> GQQVCPNYVMLRSSVTTKVVRNVVEYQIRTGGFFSCLAMLRPLQYAKRERLLGQRNLERISTRDILQTRDLHSLCMPTPDAPMSNHQASTMRELICSYFKVDHADGLKYIPMDERYSPSSLARLFTMGMAGLHITTEPSYKRVPIMHLAADLDCMTLALPYMITLDGDTVVPVAPTLSAEQLLDDGLKGLACMDISYGCEVDANSRPAGDQSMDSSRCINELYCEETAEAICVLKTCLVLNCMQFKLEMDDLAHNAAELDKIQMMIPFSERVFRMASSFATIDAQCFRFCVMMKDKNLKIDMRETTRLWTRSASDDSVATSSLSISLDRGRWVAADASDARLLVFPIRV

The mammalian orthoreovirus (reovirus) σNS protein is required for formation of replication compartments that support viral genome replication and capsid assembly. In the case of mammalian orthoreoviruses, two nonstructural proteins, σNS and µNS, initiate VF formation, and σNS recruits viral RNAs into these compartments. Our crystallographic and biochemical studies reported here provide a mechanistic understanding of how σNS forms filamentous assemblies by linking dimeric units through domain-swapping interactions of the N-terminal arms and further how such a multimeric association is required for the RNA helix-destabilizing and RNA-annealing activities of σNS. An important finding from our studies is that mammalian orthoreovirus σNS has RNA helix-destabilizing and RNA-annealing activities without requiring a metal ion or ATP, which makes this protein an RNA chaperone.

To provide additional evidence for the role of domain-swapping interactions of the N-terminal arms in forming oligomeric assemblies, we engineered a deletion construct, σNS-ΔN17, by truncating the N-terminal 17 residues of the protein. The σNS-ΔN17 mutant formed dimers in solution and also crystallized in the presence of bile acid derivatives. The σNS-ΔN17 crystal structure determined using molecular replacement showed a dimer formed by a central core identical to that in the structures of Se-Met or native σNS-R6A with two bound bile acid moieties. As expected, no helical packing was observed in the crystal structure. Therefore, the structure of σNS-ΔN17 suggests that the N-terminal arm and the core of WT σNS operate as independent structural units, and removing the N-terminal arm does not alter the dimeric association of the core. Furthermore, the σNS-ΔN17 structure showed that bile acid derivatives bind to the same location in σNS as the N-terminal arm in the σNS-R6A structure, suggesting that this location in the σNS core domain has an affinity for cholesterol-like molecules and that binding to such molecules disrupts filamentous helical assemblies by competing with the binding of the N-terminal arms. As anticipated, RNA-binding capacity and oligomer formation of σNS were abolished by the removal of the N-terminal 17 residues and, concomitantly, the σNS-ΔN17 mutant did not have RNA chaperone activity. From our studies, deletion of the N-terminal arm of σNS abrogates dimer-dimer interactions and precludes the formation of higher-order multimers.>MARRILVVEDEAPIREMVCFVLEQNGFQPVEAEDYDSAVNQLNEPWPDLILLDWMLPGGSGIQFIKHLKRESMTRDIPVVMLTARGEEEDRVRGLETGADDYITKPFSPKELVARIKAVMRRISPMA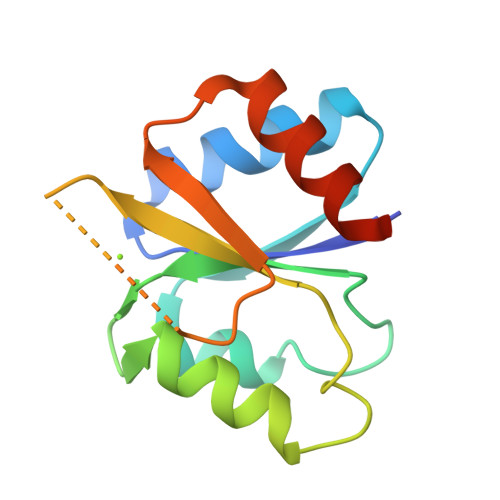[3x]> LARVAEALGSSEQALRLIVSILMGYPFALFQRYFLFQKETYLIHLYNVFTGLSIAYFNFGMQFFHSLLCVLIQFLILRLMGRTVTAVFTTFVFQMTYLMAGYYFTATEHYDIKWTMPHCVLTLKLIGLAIDYYDGGKDPELLTPEQRRFAVRGVPTLLEVSGFSYFYGAFMVGPQFSMTDYQKLAKGEMTDVPGQRPNSFVPALKRLSLGLLFLVTYTLSSPYISEEYLISDDYMEKPFWFRCGYILVWGKIILYKYVTCWLVTEGVCILVGLGYNGNDQNGKPVWDACANMKVWLYETTPLFTGTIASFNINTNAWVARYVFKRLKFLGNKLLSQALALFFLAIWHGLHSGYLVCFQMELLIVIVERQVINLVRDSPTLSTLASITALQPIFYVLQQTNHWMFMGYSLVPFCLFTWDKWMKVYKSIYFLGHVLFFTLLLVLPYIRKL

The re-acylation is catalyzed by lysophosphatidylcholine acyltransferase (LPCAT) and among the four LPCAT members in human, the LPCAT3 preferentially introduces polyunsaturated acyl onto the sn-2 position of lysophosphatidylcholine, thereby modulating the membrane fluidity and membrane protein functions therein. Combining the x-ray crystallography and the cryo-electron microscopy, we determined the structures of LPCAT3 in apo-, acyl donor-bound, and acyl receptor-bound states. A reaction chamber was revealed in the LPCAT3 structure where the lysophosphatidylcholine and arachidonoyl-CoA were positioned in two tunnels connected near to the catalytic center. The structural and functional analysis provides the basis for the re-acylation of lysophosphatidylcholine and the substrate preference during the reactions.

Overall, cLPCAT3core crystallized in the monomeric form, and residues 42–459 were resolved in each protomer. The helices in N- and C-wings tilt to converge at the cytoplasmic side and thus form a large cavity embedded in the exoplasmic leaflet of the ER membrane and open to the ER lumen, which is filled with loops and Ha-f. The structural analysis using the program HOLLOW40 shows a “T”-shape inner chamber enclosed by TM helices and Hd-f. In general, this T-shape chamber is composed of a “horizontal” tunnel parallel to the ER membrane and proximal to the cytoplasmic side, which connects with a “vertical” tunnel at the middle point. The horizontal tunnel extends from the N-wing to the C-wing and its tip in the N-wing ends at a gap between TM1 and 6, which opens laterally to the lipid environment of the ER membrane and thus might represent a potential gate for the chamber (hereafter lateral gate). The vertical tunnel is perpendicular to the horizontal tunnel and extends to the ER lumen, with a small “side pocket” extruding in the middle. The T-shape chamber is empty in the crystal structure and the analysis on the Fo-Fc electron map failed to identify any non-proteinous density. Only crystals of substrate-free cLPCAT3 can diffract to a resolution beyond 4 Å and co-crystallization of cLPCAT3 with either LPCs or acyl-CoAs failed to generate crystals capable of diffracting to 5 Å. The cryo-EM map analysis on cLPCAT3/araCoA revealed the non-protein electron density sandwiched by cLPCAT3 protomers and two 1,2-dioleoyl-sn-glycero-3-phosphocholine (DOPC) molecules were well modeled into the large blobs of electron density. This non-contact dimerization might be mediated by those intermediary lipid molecules and the relatively harsh detergents used in the crystallization trial deprived the cLPCAT3 of the lipids bound, resulting in the monomeric biological unit in cLPCAT3 crystals. Although crystallized as a monomer, the cLPCAT3 forms dimer in both membrane-bound state and subsequent EM analysis in detergents.4-[(5,5,8,8-tetramethyl-5,6,7,8-tetrahydronaphthalen-2-yl)carbamoyl]benzoic acid 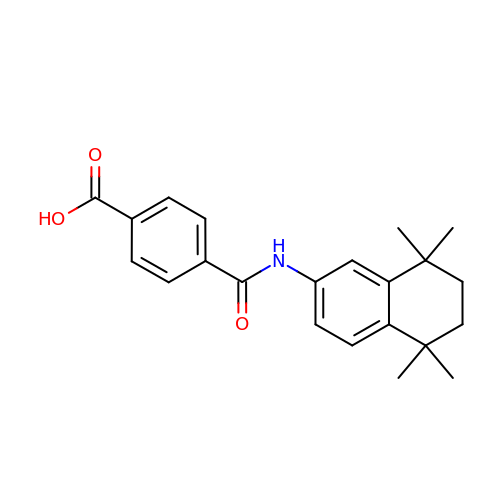| C22 H25 N O3 | MUTNCGKQJGXKEM-UHFFFAOYSA-N>MDKKQVTDLRSELLDSRFGAKSISTIAESKRFPLHEMRDDVAFQIINDELYLDGNARQNLATFCQTWDDENVHKLMDLSINKNWIDKEEYPQSAAIDLRCVNMVADLWHAPAPKNGQAVGTNTIGSSEACMLGGMAMKWRWRKRMEAAGKPTDKPNLVCGPVQICWHKFARYWDVELREIPMRPGQLFMDPKRMIEACDENTIGVVPTFGVTYTGNYEFPQPLHDALDKFQADTGIDIDMHIDAASGGFLAPFVAPDIVWDFRLPRVKSISASGHKFGLAPLGCGWVIWRDEEA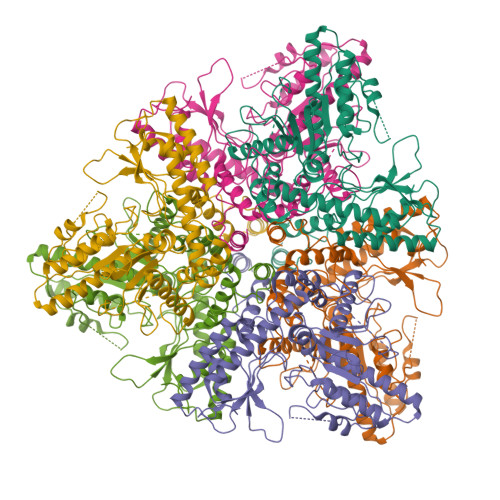LPQELVFNVDYLGGQIGTFAINFSRPAGQVIAQYYEFLRLGREGYTKVQNASYQVAAYLADEIAKLGPYEFICTGRPDEGIPAVCFKLKDGEDPGYTLYDLSERLRLRGWQVPAFTLGGEATDIVVMRIMCRRGFEMDFAELLLEDYKASLKYLSDHPKLQGIAQQNSFKHT[6x]>MRPRLWEGQDVLARWTDGLLYLGTIKKVDSAREVCLVQFEDDSQ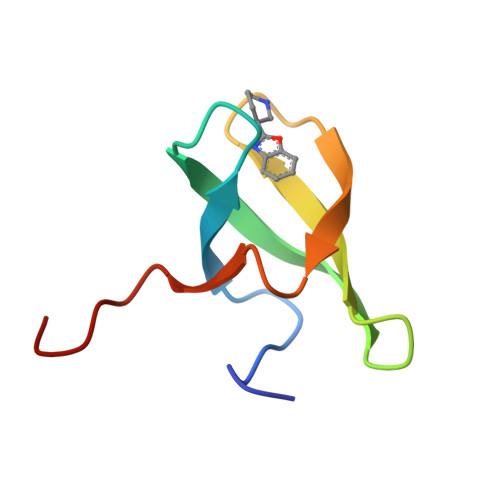FLVLWKDISPAALPGEE[3x]> MGSSHHHHHHSSENLYFQGAMKLIIAGKNNIAVDVTKWIIKTISDIELYSVCNENDHGNDSFQLSFKKFC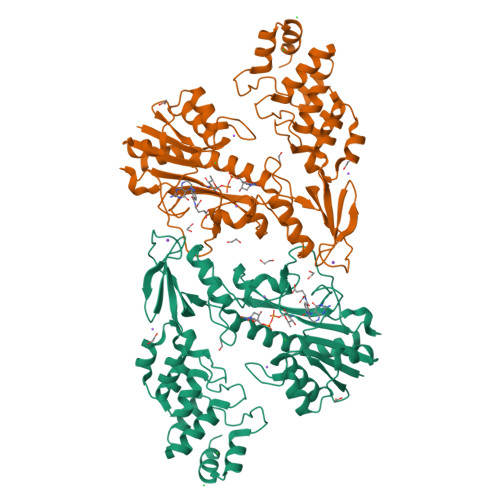IQFNIPIISLEDAYHLEDAIFLSLEFDKIIHPSKFTHNRIFNIHFSYLPAYKGMYTSAWPILNNEQESGVTLHKIDHGIDTGAIIDQQKFPLDIEETAKTLYLKYIKIGTEIVIKNLPALISGNYSIVEQSAIKSSYYSKKSIDYKNLMIDLNKTAHEILQQIRAFTFRDYQLPRIDDIDIFHGEILSSKSLSKPGTILEKNNYHLILSTIDYDIKLYSDNFDEILTACEDKSPEFISKLLKTENILFEKNHLGASPIIIAAYHGNMDVIEWLVSKGVNINDRNYKGTTVAMYFKDYMLRSGNYTGLENLINLGLDLFLKDNEGLSVFDYMRKNKNIELFNFMSTFN> VNSLSSPNSLFTGHSLEVGPSYRLIMQ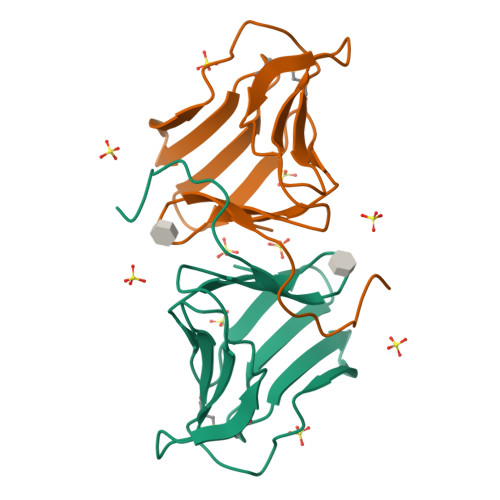GDCNFVLYDSGKPVWASNTGGLGSGCRLTLHNNGNLVIYDQSNRVIWQTKTNGKEDHYVLVLQQDRNVVIYGPVVWATGSGPA>MNERLKEKLAVLPEQPGCYLMKDKHGTVIYVGKAKSLKERVRSYFTGTHDGKTQRLVEEIADFEYIVTSSNAEALILEMNLIKKHDPKYNVMLKDDKSY[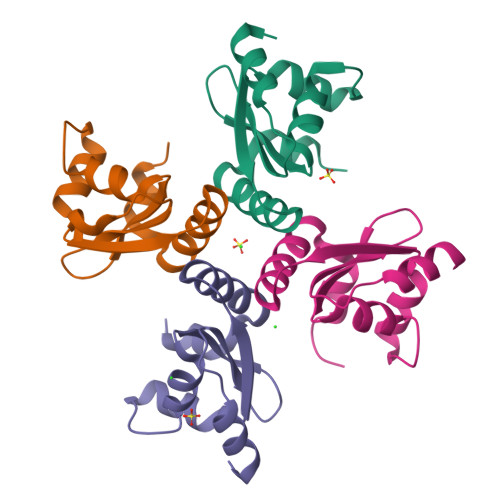4x]> GTSQVINGEMQFYARAKLFYQEVPATEEGMMGNFIELSSPDIQASQKFLRKFVGGPGRAGTDCALDCGSGIGRVSKHVLLPVFNSVELVDMMESFLLEAQNYLQVKGDKVESYHCYSLQEFTPPFRRYDVIWIQWVSGHLTDKDLLAFLSRCRD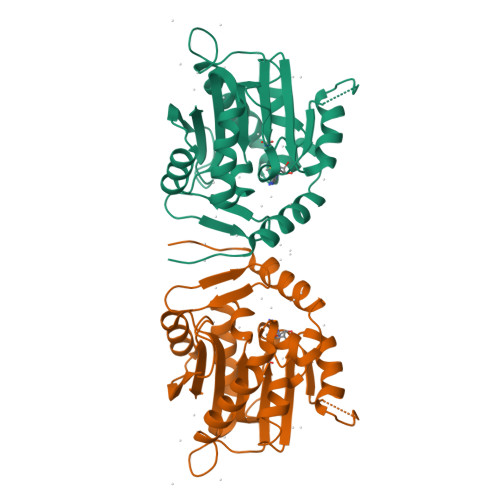GLKENGIIILKDNVAREGCILDLSDSSVTRDMDILRSLIRKSGLVVLGQEKQDGFPEQCIPVWMFALH1-deoxy-1-{[(5S)-2,6-dioxo-5-(propanoylamino)-1,2,5,6-tetrahydropyrimidin-4-yl]amino}-D-ribitol 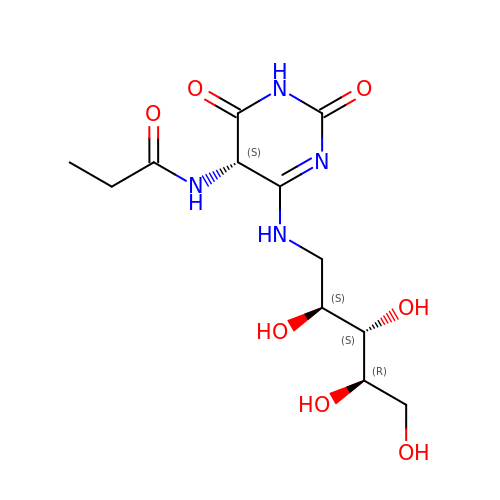| C12 H20 N4 O7 | NPNFNBTUUJYCDD-FAYXRDSDSA-N> VTCVS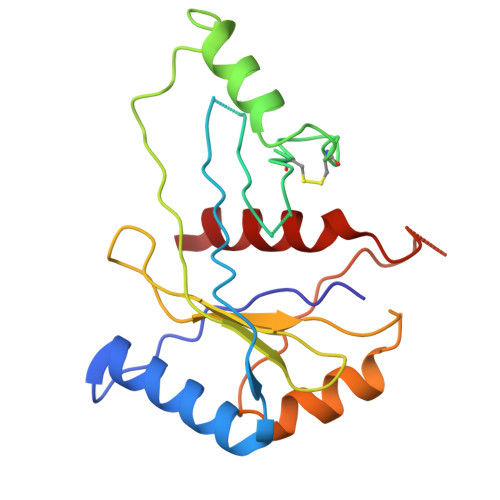QMPVAEGKSLQQTVELLTKKLEMLGAEKQGTFCVDCETYHTAASTLGSQGQAGKLMYVMHNSEYPLSCFALFENGPCLIADTNFDVLMVKLKGFFQSAKASKIETRGTRYQYCDFLVKVGTVTMGPSARGISVEVEYGPCVVASDCWSLLLEFLQSFLGSHAPGAPTVFGNRHDAVYGPADTMIQYMELFNKI~{N}4-(phenylmethyl)-~{N}4-[2-[3-(2-piperazin-1-ylpyrimidin-5-yl)phenyl]phenyl]pyrimidine-2,4-diamine | C31 H30 N8 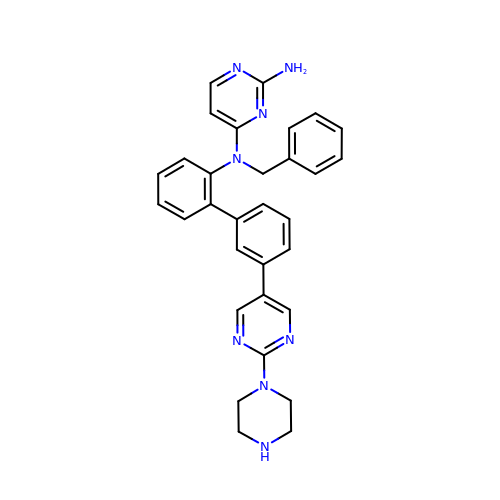| FRBABIFCTILEGV-UHFFFAOYSA-N> IPVIEPLFTKVTEDIPGAEGPVFDKNGDFYIVAPEVEVNGKPAGEILRIDLKTGKKTVICKPEVNGYGGIPAGCQCDRDANQLFVADMRLGLLVVQTDGTFEEIAKKDSEGRRMQGCNDCAFDYEGNLWITAPAGEVAPADYTRSMQEKFGSIYCFTTDGQMIQVDTAFQFPNGIAVRHMNDGRPYQLIVAETPTKKLWSYDIKGPAKIENKKVWGHIPGTHEGGADGMDFDEDNNLLVANWGSSHIEVFGPDGGQPKMRIRCPFEKPSNLHFKPQTKTIFVTEAENNAVWKFEWQRNGKKQ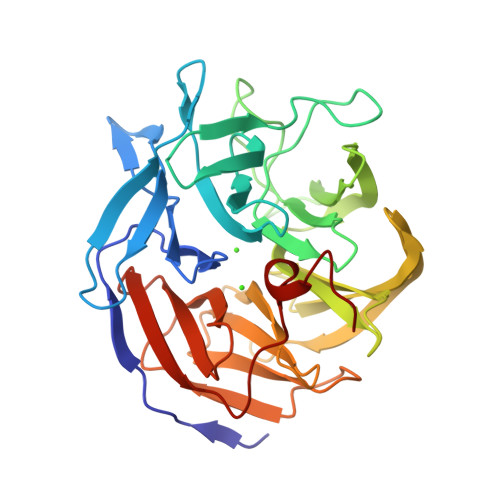YCETLKFGIF> GSHMVKEINESIFDEEIKTSGEPVIVDFWAPWCGPSKMLGP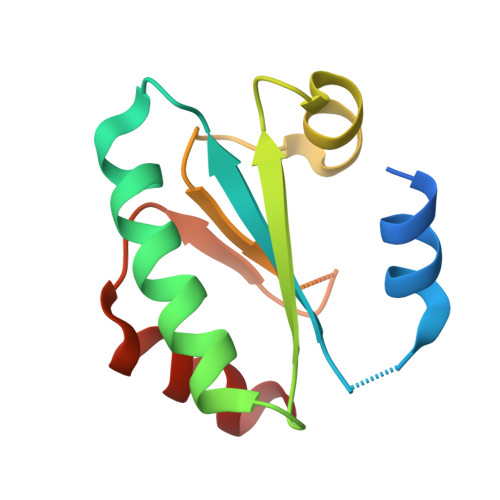IIDELSEDLDGKAKFTKVNVDENPGIASKFGIASIPTVMIFKDGNPVETLVGFRPKQSITASIEKHM>QDLMASGNTTVKATFGKDSSVVKWVVLAEVLVGAVMYMMTKNVKFLAGFAIISVFIAVGMAVVGL[75x]

Conjugative pili are widespread bacterial appendages that play important roles in horizontal gene transfer, in spread of antibiotic resistance genes, and as sites of phage attachment. The pilus is a polymer of the VirB2 protein (or pilin). The structures of the pED208 and F pilus are very similar, with overall dimensions of 87 Å in diameter and an internal lumen of 28 Å in diameter. Thus, selective binding of PG to pilins occurs in both F and pED208 pili, and thus, the F family of pili are polymers of a selective and stoichiometric protein-PG complex unit.

During the process of helical reconstruction, as the resolution was increased, an additional separate density became clearly visible and readily interpretable as a phospholipid. For the F pilus, it became apparent during the process of helical reconstruction that two populations of filaments were present, differing slightly in the rise between subunits (see below). Instead, two 5.0 Å resolution electron density maps were generated for the two F pilus populations. For pED208, the angle between adjacent subunits is 28.2° and the rise is 12.1 Å, while for the two F pilus structures, the helical parameters were 27.9° with a rise of 13.2 Å and 28.1° with a rise of 12.5 Å, respectively. Superposition of the structures of pED208 and F TraA reveals very similar overall structures (root-mean-squared deviation in Cα positions between pED208 and F [13.2 Å rise] of 1.4 Å and between pED208 and F [12.5 Å rise] of 1.5 Å) with slightly different boundaries for secondary structures. Also, the TraA pilin structures in the two F pilus forms are virtually identical (root-mean-squared deviation in Cα positions of 0.7 Å). Thus, with the structures and helical parameters of the two F pilus forms being so similar, functional differences between them are unlikely to arise but cannot be excluded. The amino acid sequences of both the orthologous pED208 and F pilus TraA pilin are similar, except for the F pilin N terminus, which is 4 amino acids (aa) longer. This longer N terminus could not be traced in the F pilus density maps and thus must be disordered. Indeed, the presence of phospholipid in the F pilus was also confirmed by MS; however, this time a PG species, PG 33:1 (16:0, ΔC17:0), was the major phospholipid observed in the F pilus after PLA2 treatment.>[2x]MTAAPAALHDRALHLLQTIWGYPAFRGVQGEIVQQVAEGGNALVLMPTGGGKSLCYQLPSLLRPGTGIVVSPLIALMKD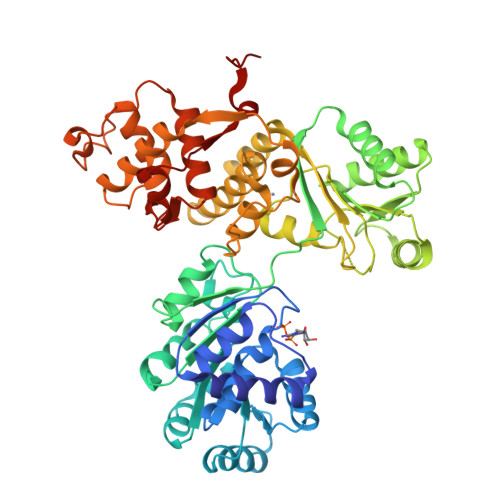QVDTLRQNGVRAAFLNSTLLPHEAREVEDALLRGDLDLLYVAPERLLMPRTLDLLERAPVALFAIDEAHCVSQWGHDFRPEYQQLSVLAERFPELPRVALTATADERTRADIKSVLRLEDAPQFVSSFDRPNIQYRVGLKDSPKTQLLHFIREEHPGDAGIVYCLSRKSVEETAKWLQAQGIDALAYHAGLSSTERNNVQERFLNEEGVIVCATVAFGMGIDKPNVRFVAHLDLPKSMEGYYQETGRAGRDGLPSTAWMVYGLSDVVNVRRMLAQSDAPEEVKRVEASKLDALLTYCEAATCRRQVLLHYFGEELSEPCGNCDVCLNPPRVRDLTREAQMALSATIRTGNRFGAAHLTDVLLGRETDKVLAQGHHQLPTFGVGKEHDEKLWRSVLRQLVSLGYLSADDHFGLRATGKSRGILKEGQKLLLREDTLLPGLEHHHHHH>HHHHHHSGRSVANQANLIDNKRELEQHALVPYAQGKSIHQLFEEQAEAFPDRVAIVFENRRLSYQELNRKANQLARALLEKGVQTDSIVGVMMEKSIENVIAILAVLKAGGAYVPIDIEYPRDRIQYILQDSQTKIVLTQKSVSQLVHDVGYSGEVVVLDEEQLDARETANLHQPSKPTDLAYVIYTSGTTGKPKGTMLEHKGIANLQSFFQNSFGVTEQDRIGLFASMSFAASVSEMFMALLSGASLYILSKQTIHDFAAFEHYLSENELTIITLPPTYLTHLTPERITSLRIMITAGSASSAPLVNKWKDKLRYINAYGPTETSCSATI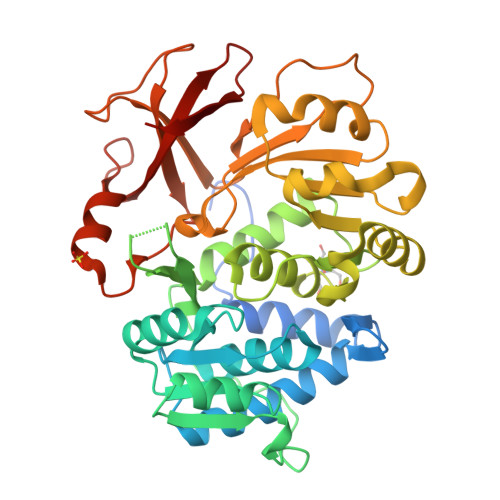WEAPSNQLSVQSVPIGKPIQNTHIYIVNEDLQLLPTGSEGELCIGGVGLARGYWNRPDLTAEKFVDNPFVPGEKMYRTGDLAKWLTDGTIEFLGRI[2x]> NLGLDCDEHSSESRCCRYPLTVDFEAFGWDWIIAPKRYKANYCSGQCEYMFMQKYPH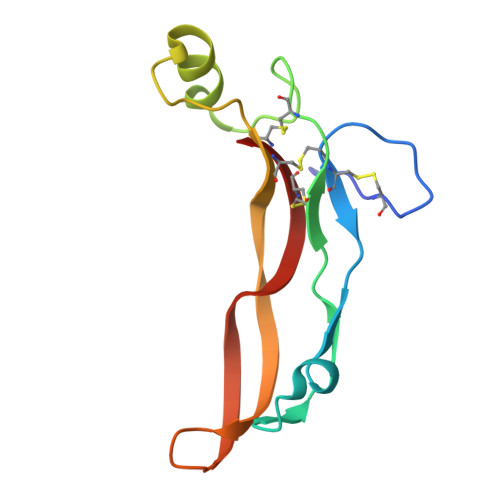THLVQQANPRGSAGPCCTPTKMSPINMLYFNDKQQIIYGKIPGMVVDRCGCS>MGSSHHHHHHSSGAGVLTIGCREDSTTFDPIKSAQNRDTWVFANVYDTLVRVDNLGTKMEPGLAESWDISKDGLTYTFKLREAKFSDGSPITAEDAAFSLLRIRDNKASLWSDPFSLINTAKATDPKTLVVTLKTPAVAFLSQLASPTVSILSEKAMTKMGEDAYAENPVTSGAFTVDEWRKGDRVILKKNPNFWQAKNVSLDGVEWVSVTDDNTRMRMVQNNELDTAIFVPFSRVEELKKDKNVVIHSDPSTREDHLLINHEHGLLAKPEVRQALDMAIDKQSLVKTATYGQGTVAYSYIPKGSLYHYANNLQRPYDPAAAKKLLADAGAKDLKLNYVVNAGNEADEQIAV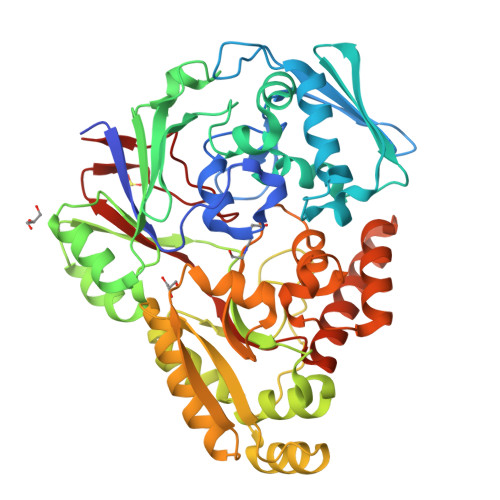IIKDQLAKVGVTANLQKVDPTQSWQMLVDGTYDISVMYWTNDILDPDQKTTFVLGHDTNQNYMTRYKNDQVKALVAAARIEADPAKREQMYIDLQKLAKQDVNWIDLYYSPYINISRKNVSNFLQNPLGRFTLEEVVKN[2x]>[2x]DYTEKQAVPISVPRYKHVEQNGEKFVVYNVYMAGRQLCSK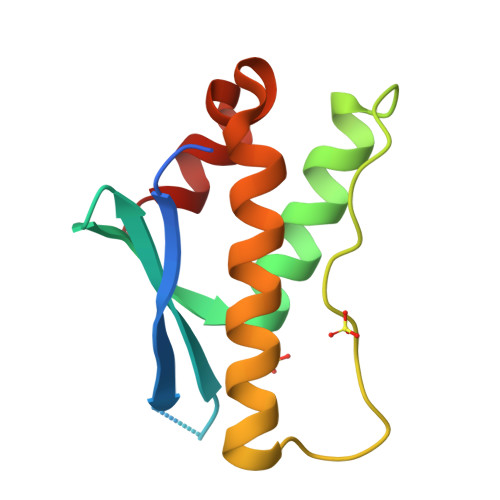RYREFAILHQNLKREFANFTFPRLPGKWPFSLSEQQLDARRRGLEEYLEKVCSIRVIGESDIMQEFLSES> ESPMSSDKGRNRWSRYIGSIHTMGFATRPTVKPVPIGSRLGFKKSVPKDLPLGKSLQHQHCSHLVRLIDTSQDRELGRMPEDVARILYPLLDYSEQVSLEPYLLINNGKRFSVGDNIYIRIDCYLTSQAFVRIEGGSILNKSFINDHGMDTRQLHRAGAIMALFDAINIQPVYGDTKNEMIPNYQENTVSSSQFQDEALNINQLKSFYRITQSAASLQNLPETTPDESLFKLQLRRYQKQSLSWMLKREYEYSHLSEKAAEVSIDGNSMNPLWKKFRWPSNSKQGTPNHEDDCFFYANLYTGEFSIEKPVIKTIINGGILADEMGLGKTISALALICTASYDEAHEKKIESTKKPSMKEMSSQVDSSPLRHSQHKHDTYAYRTTLIVVPMSLLNQWQSEFEKANKDLKKRCEIYYGNNIKDLRAYVLGPNAPSVIITTYGIIQSE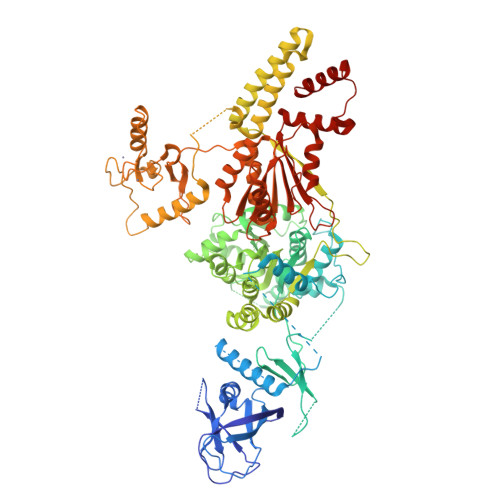YGRTSTSGLFNVVFFRIILDEGHTIRNRSTRTSKAVIALRSSRKWILTGTPIINRLDDLFSLVQFLNLEPWSHINYWKRYVSVPFEKGNYAQAFDVINAVLEPVLLRRTKNMKDVDGKPLVSLPPKEVIVEKLQLSSSEKRVYQSMLEDAENSVKEGLAKGDLLKNYTNILVHILRLRQVCCHLDLLKKTPDLGDPDLEDLENSTQNISSILMPKNIKSPKSSISQDKLDALSANFRDIHSASEQLPSFECAICTTECIEPLSAVSITECLHTFCEPCLAEYIEFQQNKKLSINCPYCRMPISEANVLKLKEPIDAERGYELISFHSHFQSTKIKALLRHLKQIQETSPGEQIIVFSQFSSFLDILEIELRSHLPRDQVIIYKFDGRLDMKERTRILEQFHDKDLSCIKLLLLSLKTGGVGLNLTCASRAFMMDPWWSPGMEDQAIDRIHRIGQQQTVKVVRFIIDNSVEEKMLRIQERKRMLGDIVEGDEAERRQKRIEEIQMLFQ pmcThe BEN (BANP, E5R, and NAC1) domain is a ∼100-residue protein domain found in metazoans and viruses, but missing in nematodes and urochordates. There are nine BEN domain–containing transcription factors in the human genome, i.e., BANP, BEND2-7, and NAC1/2. The BEN domain-containing transcription factors regulate transcription by recruiting chromatin-modifying factors to specific chromatin regions via their DNA-binding BEN domains. Further structural analysis revealed that although all these BEN domains bind their target DNAs mainly through the insertion of the C-terminal α5 helix into the major groove of DNA, the residues of the α5 helices involved in the base interactions vary from one to another, explaining why they exhibit distinct DNA sequence preference.

To further investigate the role of cytosine methylation in BEN domain binding, we successfully obtained the structures of the BEND6 BEN domain in complexes with the CGCG motif and CGmCG motif containing DNAs, respectively. Structural analysis revealed that the BEND6 BEN domain adopted a canonical α-helical architecture but lacked the N-terminal β-hairpin compared to that of the BANP BEN domain. Like the BANP BEN domain as well as other reported BEN domains, the α5 helix of BEND6 inserted into the major groove of DNA, while a longer Loop 1 stepped into the minor groove of DNA, which together contributed to the electrostatic interactions with the DNA. In the BEND6-CGCG DNA structure, the side chain of K265 from the α5 helix formed two hydrogen bonds with the bases of G3′ and A4′, respectively, while the side chain of N261 from the α5 helix made hydrogen-bonding interactions with the base of G5′. The side chains of R254 from the α5 helix and S216, T218 from the Loop 1 formed four hydrogen bonds with the base of G7′. In addition, the side chain of S217 also made two hydrogen bonds with the base of G8. Moreover, the side chains of Q258, N261, and N262 formed water-mediated hydrogen bonds with the bases of C3 and C5, respectively. In addition to these base interactions, the side chains of K191, N194, T212, K225, R253, Q258, K259, and N262 formed several hydrogen bonds and salt bridges with the DNA backbone. Interestingly, the side chain of R254 adopted two conformations, one of which made interactions with the base and the other made interactions with the DNA backbone. The results showed that mutating R254, N261, and K265 to alanine individually reduced the binding of the BEND6 BEN domain with the CGCG DNA by ∼2-6-fold, suggesting that these residues played a role in DNA binding.

> GDEKQFQIEKWQIARCNKSKPQKFINDLMQVLYTNEYMATHSLTGAKSSTSRDKAVKPAMNQNEVQEIIGVTKQLFPNTDDVSIRRMIGQKLNNCTKKPNLSK>[2x]ASAWPEEKNYHQPAILNSSALRQIAEGTSISEMWQNDLQPLLIERYPGSPGSYAARQHIMQRIQRLQADWVLEIDTFLSQTPYGYRSFSNIISTLNPTAKRHLVLACHYDSKYFSHWNNRVFVGATDGAVPCAMMLELARALDKKLLSLKTVSDSKPDLS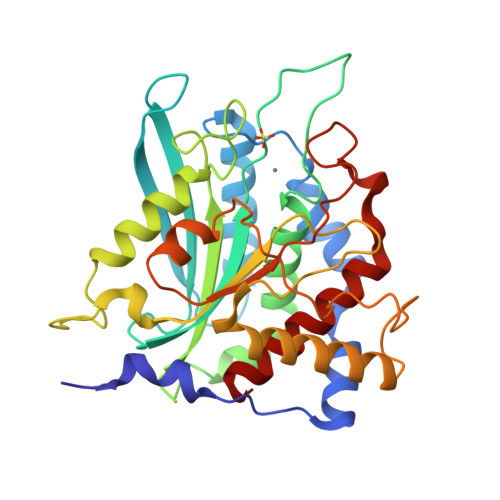LQLIFFDGEEAFLHWSPQDSLYGSRHLAAKMASTPHPPGARGTSQLHGMDLLVLLDLIGAPNPTFPNFFPNSARWFERLQAIEHELHELGLLKDHSLEGRYFQNYSYGGVIQDDHIPFLRRGVPVLHLIPSPFPEVWHTMDDNEENLDESTIDNLNKILQVFVLEYLHL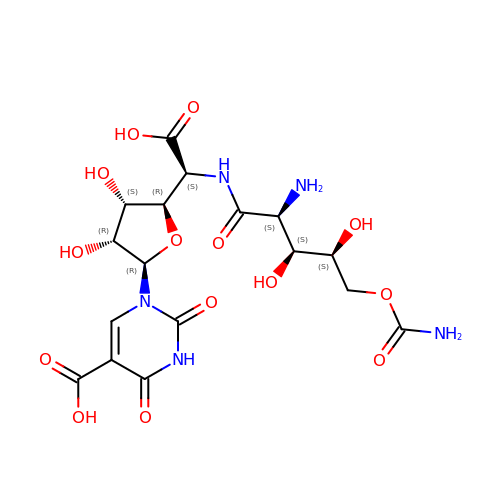1-{(2R,3R,4S,5R)-5-[(S)-{[(2S,3S,4S)-2-amino-5-(carbamoyloxy)-3,4-dihydroxypentanoyl]amino}(carboxy)methyl]-3,4-dihydroxyoxolan-2-yl}-2,4-dioxo-1,2,3,4-tetrahydropyrimidine-5-carboxylic acid (non-preferred name) | C17 H23 N5 O14 | JPFWJDMDPLEUBD-ITJAGOAWSA-N>[2x]MNAAAVTPPPEKFNFAEHLLQTNRVRPDKTAFVDDISSLSFAQLEAQTRQLAAALRAIGVKREERVLLLMLDGTDWPVAFLGAIYAGIVPVAVNTLLTADDYAYMLEHSRAQAVLVSGALHPVLKAALTKSDHEVQRVIVSRPAAPLEPGEVDFAEFVGAHAPLEKPAATQADDPAFWLYSSGSTGRPKGVVHTHANPYWTSELYGRNTLHLREDDVCFSAAKLFFAYGLGNALTFPMTVG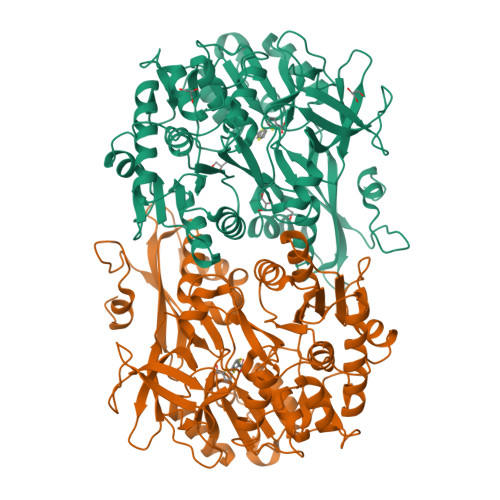ATTLLMGERPTPDAVFKRWLGGVGGVKPTVFYGAPTGYAGMLAAPNLPSRDQVALRLASSAGEALPAEIGQRFQRHFGLDIVDGIGSTEMLHIFLSNLPDRVRYGTTGWPVPGYQIELRGDGGGPVADGEPGDLYIHGPSSATMYWGNRAKSRDTFQGGWTKSGDKYVRNDDGSYTYAGRTDDMLKVSGIYVSPFEIEATLVQHPGVLEAAVVGVADEHGLTKPKAYVVPRPGQTLSETELKTFIKDRLAPYKYPRSTVFVAELPKTATGKIQRFKLREGVLG The retinoblastoma tumor suppressor (Rb) is a multifunctional protein that primarily regulates the cell cycle but also has roles in cellular differentiation, DNA damage response, and apoptosis. Essential functions of Rb occur through its pocket domain, which is necessary for regulating binding interactions with E2F transcription factors and transcription repressors that bind via an LxCxE motif. The pocket domain is the most highly conserved region of the multidomain protein, as well as the most frequent site of mutations. Protein X-ray crystallography of four missense variants reveals how mutations destabilize the protein fold and inhibit E2FTD or LxCxE binding.

Missense variants within the hydrophobic core of subdomain B, such as I703F, I703V, M695I, and M704V, show reduced stability and temperature-sensitive binding to E2F1TD and E7LxCxE. To understand how these mutations induce such effects, we crystallized M704V. The crystal structure of M704V reveals changes to the packing of the hydrophobic core of subdomain B. Specifically, M704V introduces new steric bulk in the form of valine’s second gamma carbon. This forces alternative rotamers of F684 and L688 through changes to a van der Waals contact network. Although, it was not clear from the structure of M704V why E2F1TD and E7LxCxE binding are affected by this variant, since the mutation site is distant from binding sites. While Rb’s M704V mutation alters the hydrophobic core energetic ground state by reconfiguring several buried residues, these changes must also have structural consequences that extend beyond the hydrophobic core. Additional experiments are needed to elucidate the structural mechanisms through which changes to core packing translate to E2FTD- and E7LxCxE-binding inhibition by some RbP variants.

>[2x]GEFNTIQQLMMILNSASDQPSENLISYFNNCTVNPKESILKRVKDIGYIFKEKFAKAVGQGCVEIGSQRYKLGVRLYYRVMESMLKSEEERLSIQNFSKLLNDNIFHMSLLACALEVVMATYSRSTSQNLDSGTDLSFPWILNVLNLKAFDFYKVIESFIKAEGNLTREMIKHLERCEHRIMESLAWLSDSPLFDLIKQSKDREGPTDHLESACPLNLPLQNNHTAADMYLEPVRAPKKKSTSLSLFYKKVYRLAYLRLNTLCERLLSEHPELEHIIWTLFQHTLQNEYELMRDRHLDQIVMCSMYGICKVKNIDLKFKIIVTAYKDLPHAVQETFKRVLIKEEEYDSIIVFYNSVFMQRLKTNILQYASTRPPTLAPIPHIPRSPYKFP> MDPDELPLDEHCERLPYDASKWEFPRDRLNLGKPLGRGAFGQVIEADAFGIDKTATCRTVAVKMLKEGATHSEHRALMSELKILIHIGHHLNVVNLLGACTKPGGPLMVIVEFCKFGNLSTYLRSKRNEFVPYKDLYKDFLTLEHLICYSFQVAKGMEFLASRKCIHRDLAARNILLSEKNVVKICDFGLARDIYKDPDYVRKGDARLPLKWMAPETIFDRVYTIQSDVWSFGVLLWEIFSLGASPYPGVKIDEEFCRRLKEGTRMRAPDYTTPEMYQTMLDCWHGEPSQRPTFSELVEHLGNL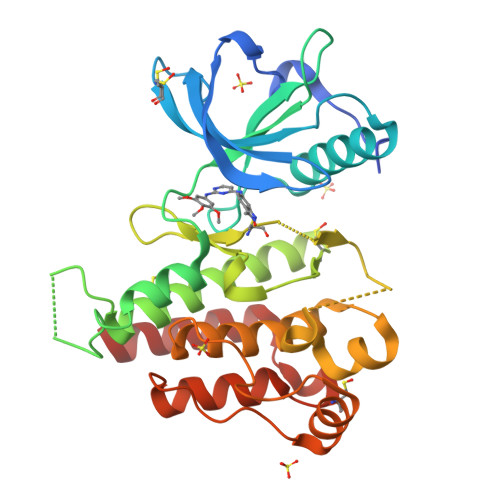LQANA Toll-like receptor 4 (TLR4), a superfamily of LRR proteins, is the principal receptor mediating innate immune responses against infections by Gram-negative bacteria. In this process, myeloid differentiation protein 2 (MD2) recognizes various lipopolysaccharides (LPSs) released from the Gram-negative bacteria, forming a complex with LPS at its hydrophobic pocket. In an attempt to prevent the systemic immune response caused by LPS, a TLR4 decoy receptor was constructed by combining LRR modules from the TLR4 ectodomain and VLR. The constructed decoy receptor was shown to attenuate the TLR4-mediated signaling process by trapping MD2, implicating a potential therapeutics for bacteria-induced sepsis and inflammation.

Changing phenylalanine at position 63 was likely to form a hydrophobic interaction with Ile-66 of MD2 in the crystal structure of the decoy receptor/MD2 complex. Phe-63 was substituted for tryptophan and leucine for the interaction with Ile-66 in MD2. From the structure of the F63W and V134L mutants, it was expected that hydrophobic interactions would increase by introducing a residue with a larger hydrophobic side chain. The F63W mutant displayed increases in the Coulomb interaction and LJ potential by 17.08 and 11.02 kJ/mol, respectively, indicating a significant enhancement in the hydrophobic interaction, as expected. Trp-63 concurrently contributed to an increase in the charge interaction via additional hydrogen bonding with the residues on MD2. The crystal structures of the selected single mutants as apo and complexed with MD2 provided detailed information on the interaction modes of the residues at the interface and the contribution of mutated residues to binding affinity. Superposition of the mutants on the wild-type revealed that their original backbone structures were retained, which represents the structural characteristics of repeat proteins.

> GSPCVEVVPNITYQCMELNFYKIPDNLPFSTKNLDLSWNPLRHLGSYSFFSFPELQVLDLSRCEIQTIEDGAYQSLSHLSTLILTGNPIQSLALGAFSGLSSLQKLVAVETNLASLENFPIGHLKTLKELNVAHNLIQSFKLPEYFSNLTNLEHLDLSSNKIQSIYCTDLRVLHQMPLLNLSLDLSLNPMNFIQPGAFKEIRLKELALDTNQLKSVPDGIFDRLTSLQKIWLHTNPWDCSCPRIDYLSRWLNKNSQKEQGSAKCSGSGKPVRSIICPT CRISPR-Cas systems are prokaryotic adaptive immune systems and phages use anti-CRISPR proteins (Acrs) to counteract these systems. In the type I-F system, after pre-crRNA is transcribed, Cas6f processes the pre-crRNA into small crRNAs, binds it, and further assembles with one Cas8f, one Cas5f, and six Cas7f proteins to generate the crRNA-guided surveillance complex (Csy complex). AcrIF24 targets the Cas7f subunits by engaging up to five Cas7f subunits (Cas7.2f-7.6 f), sterically blocks access to the crRNA guide by the complementary target DNA, and induces non-sequence-specific DNA binding to the Csy complex. AcrIF24 forms a homodimer and further induces dimerization of the Csy complex.

During the process of structure determination, we found that the residues ranging from 73 to 135 of AcrIF24 tend to be disordered, with electronic density too weak to model the structure of this region. Therefore, we made another AcrIF24 construct (AcrIF24 Δmiddle domain, short for AcrIF24ΔMD hereafter) by deleting this region and linking the remaining two parts of the protein with a “GSGSSG” linker. We solved its crystal structure to a resolution of 2.10 Å. There is only one AcrIF24ΔMD molecule in the asymmetric unit. The structure of AcrIF24ΔMD revealed a two-domain architecture, with an extended N-terminal domain (residues 1–72, NTD) and a globular C-terminal domain (residues 136–228, CTD). The NTD comprises a five-stranded antiparallel β sheet and a bent α helix. The CTD comprises five α helices and a single 310 helix. In the structure, the two helices ranging from residue 181–198 of AcrIF24CTD (colored orange), almost perpendicular to each other, constitute an HTH motif, linked by the characteristic sharp turn (residues 189–191). In the crystal, two AcrIF24 protomers with twofold symmetry interact with each other with several hydrophobic interactions from their CTDs, extending to a length of ~113 Å. The results showed that mutating F212/H216/Y217 to either alanines or glutamates changed AcrIF24ΔMD to monomers as indicated by the assays of gel filtration chromatography.

> MNAIHIGPFSITPAARGLHYGGLPHHQWTLYYGPREMAIKTLPDSYTSSEVRDEFSDIIAEFVIDARHRYAPGSGSSGSAPPLAWITGLLPGEVLTHDAEEWRPPTSWELRHVVGEGSFTGVSGAAAAALLGMSATNFRKYTAGDSAANRQKISFAAWHYLLDRLGVKRAS> D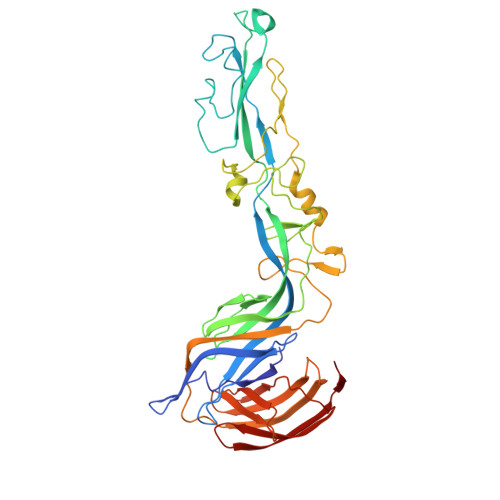PGCSELIQASSRITTCSTEGVNTKCRLSGTALIRAGSVGAEACLMLKGVKEDQTKFLKIKTVSSELSCREGQSYWTGSFSPKCLSSRRCHLVGECHVNRCLSWRDNETSAEFSFVGESTTMRENKCFEQCGGWGCGCFNVNPSCLFVHTYLQSVRKEALRVFNCIDWVHKLTLEITDFDGSVSTIDLGASSSRFTNWGSVSLSLDAEGISGSNSFSFIESPGKGYAIVDEPFSEIPRQGFLGEIRCNSESSVLSAHESCLRAPNLISYKPMIDQLECTTNLIDPFVVFERGSLPQTRNDKTFAASKGNRGVQAFSKGSVQADLTLMFDNFEVDFVGAAVSCDAAFLNLTGCYSCNAGARVCLSITSTGTGSLSAHNKDGSLHIVLPSENGTKDQCQILHFTVPEVEEEFMYSCDGDERPLLVKGTLIAID>[2x]DLNSCSMPLGMESKAISDAQITASSYF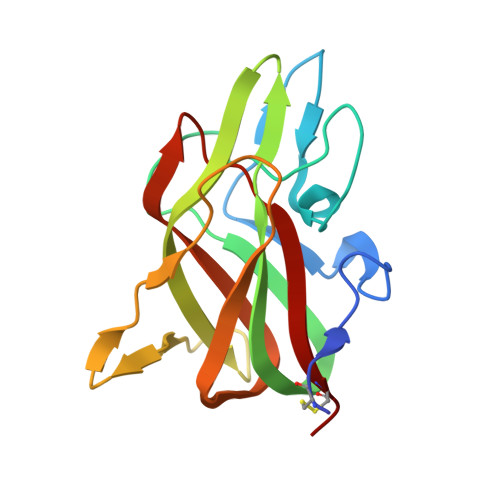TNMFATWSPSKARLHLQGRSNAWRPQVNNPKEWLQVDFQKTMKVTGVTTQGVKSLLTSMYVKEFLISSSQDGHQWTLFFQNGKVKVFQGNQDSFTPVVNSLDPPLLTRYLRIHPQSWVHQIALRMEVLGCEA> MLRRAVVALRRDALNGGSSMTLGSKGMKLSPDPHRRRMPWTAAKEYVPGVVLNAKEKMVLDGVKLVDVECVDRASQVDPLEALRATVATYEYNTSTGKNIFQLASQVEFDGRGQRFYRKEWQEGTYDKYVTLSAIDFNRDGNKGTAYGYVTFHGETTTRPVQIDFADVPGW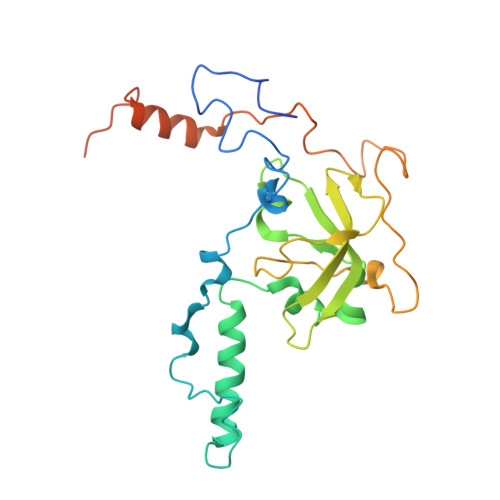HMEFRVERAVPFNAIVPPPPSIGTDVPVDPRSYRLRAYPFYDAPNPPEFVERLLKDRGVIPDSPVETTELPNESEGSDDTTRRKN> MSQAIGILELSSIAKGMELGDAMLKAAN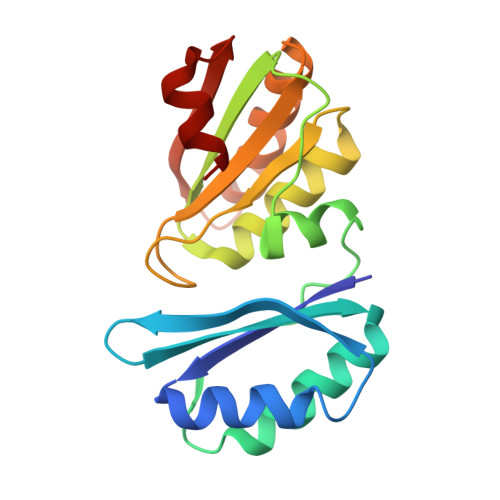VDLLVSKTISPGKFLLMLGGDLDDIILAVAVGMERAGDSLLDSEVIPDIHPSVLPAISGLNSVDKRQAVGIVETWSVAACIKAADRAVKGSNVTLVRVHMAFGIGGKCYMVVAGDVSDVNNAVTVASESAGEKGLLVYRSVIPRPHEAMWRQMVEG> MGDNLTDLPGVGPSTAEKLVEAGYIDFMKIATATVGELTDIEGISEKAAAKMIMGARDLCDLGFKSGIDLLKQ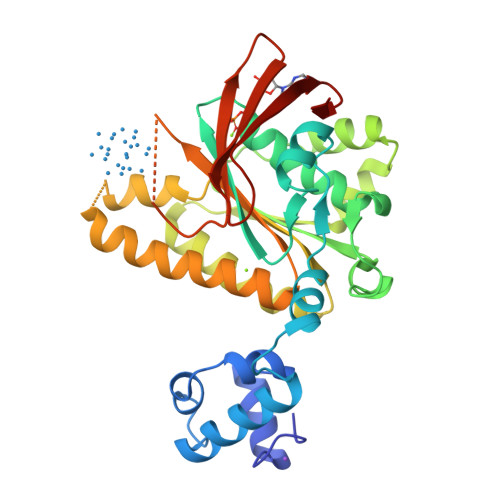RSTVWKLSTSSSELDSVLGGGLESQSVTEFAGVFGSGKTQIMHQSCVNLQNPEFLFYDEEAVSKGEVAQPKAVYIDTEGTFRPERIMQMAEHAGIDGQTVLDNTFVARAYNSDMQMLFAEKIEDLIQEGNNIKLVVIDSLTSTFRNEYTGRGKLAERQQKLGRHMATLNKLADLFNCVVLVTNQVSAKPDAFFGMAEQAIGGHIVGHAATFRFFVRKGKGDKRVAKLYDSPHLPDAEAIFRITEKGIQD> AVTHHHHHHSTGCTVGGSQTEGNMNKFGTLNFGKTSGTWNNVLTAEVASAATGGNISVTCDGTDPVDFTVAIDGGERTDRTLKNTASADVVAYNVYRDAARTN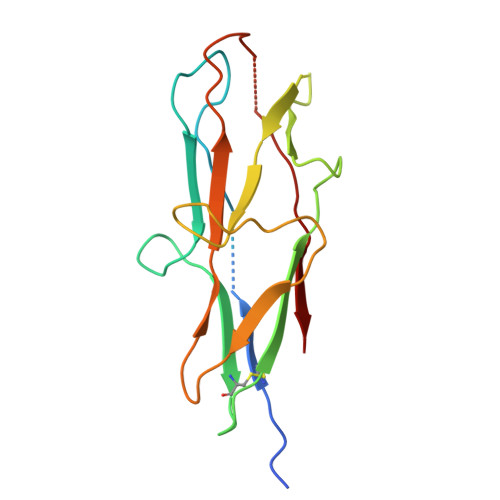LYVVNQPQQFTTVSGQATAVPIFGAIAPNTGTPKAQGDYKDTLLVTVNF> MAHHHHHHMKQKIWYTYDDIHRVIKALAEKIRNAGVKYDAMIAIGGGGFIPARMLRCFLEIPIYAVTT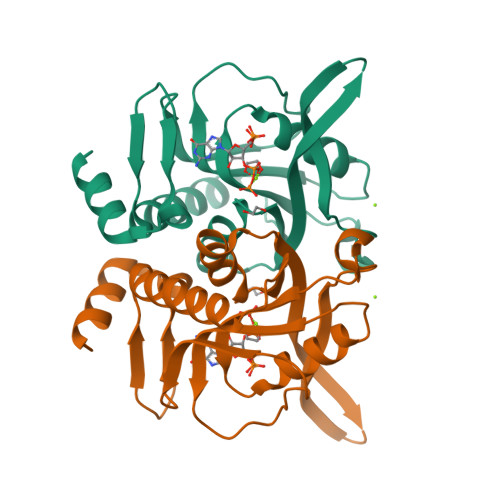AYYDSDNEGQVTEEVKKVQWLDPVPEVLRGKNVLVVDEVDDSRVTMEFCLKELLKEDFDTVGVAVLHEKIKAKAGKIPEGIPYFSGITVEDWWINYPWDALDIDEHNRLAEAGRG>MSLSAHEIRELFLSFFEKKGHTRVKSAPLVPENDPTLLFVNAGMVPFKNVFLGLEKRPYKRATSCQKCLRVSGKHNDLEQVGYTSRHHTFFEMLGNFSFGDYFKKEAIEYAWEFVTEVLKLPKEKLYVSVYKDDEEAYRIWNEHIGIPSERIWRLGEEDNFWQMGDVGPCGPSSEIYVDRGEEYEGDERYLEIWNLVFMQYNRDENGVLTPLPHPNIDTGMGLERIASVLQGKNSNFEIDIIFPLIQFGEEVSGKKYGEKFETDVALRVIADHLRAITFAISDGVIPSNEGRGYVIRRILRRAMRFGYKLGIENPFLYKGVDLVVDIMKEPYPELELSREFVKGIVKGEEKRFIKTLKAGMEYIQEVIQKALEEGRKTLSGKEVFTAYDTYGFPVDLIDEIAREKGLGIDLEGFQCELE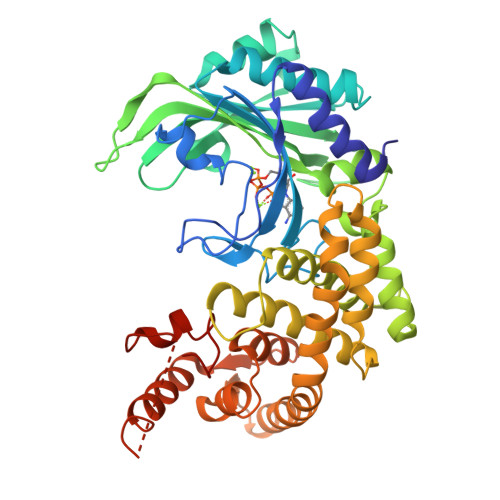EQRERARKHFKVEAKKVKPVYSHLKELGKTSAFVGAAALEHHHHHH[2x]>MADGGRVAQARALLQQCLHARLQVRPADGDAAAQWVEIRRGLVIYVCFFKGADTDLLPKMVNTLLNVKLSETETGKHVSILDLPGDVLIIPQATLGGRVKGRSMQYHSNSGKEEGSELYSQFVSLCEKAVANNTKSVEAGVAVAHGTYGNRQVLKLDTNGPYTHLIEF[2x]

Here, we describe the identification and characterization of a unique DTD-like factor, named Animalia-specific tRNA deacylase (ATD). Present in kingdom Animalia and more specifically all across phylum Chordata, ATD proofreads a critical tRNA selection error made by AlaRS. An unprecedented switch from the chiral-selective “Gly-cisPro” dipeptide in DTD to “Gly-transPro” in ATD is the key to ATD’s gaining of L-chiral selectivity. This “gain of function” through relaxation of substrate chiral specificity underlies ATD’s unique capability of correcting the error in tRNA selection.

To gain insights into ATD’s function, we solved the crystal structure of MmATD at 1.86 Å resolution. We were able to solve the structure by molecular replacement using PfDTD as the search model, despite the fact that the two share < 30% sequence identity. Structural superposition of MmATD on PfDTD and NTD from Pyrococcus abyssi (PabNTD) showed an r.m.s.d. of 1.68 Å over 141 Cα atoms and 3.34 Å over 77 Cα atoms, respectively. As is the case with DTD and NTD, ATD too is a homodimeric protein. The crystal structure of ATD revealed that its characteristic motifs (–PQATL– and –TNGPYTH–) are present at the dimeric interface like the corresponding active site motifs of DTD (–SQFTL– and –NXGPVT–). Surprisingly, MmATD’s Gly-Pro motif occurs in trans conformation, unlike DTD’s Gly-Pro motif which always exists in cis conformation as observed in 107 protomers of 19 crystal structures from 5 different organisms. In contrast, the interaction of MmATD’s Arg151 side chain with the main chain of Gly-transPro motif from the dimeric counterpart pulls the motif’s backbone outwards, thus holding the motif rigidly in trans conformation. Comparative analysis of active sites of DTD and ATD further revealed that the inward flip of ATD’s carbonyl oxygens due to trans conformation of its Gly-Pro motif has created “additional” space in its active site when compared to DTD. Strikingly, when tested with L-Ala-tRNAAla, 500 nM MmATD displayed noticeable activity. Strikingly, biochemical assays with MmATD showed significantly higher selectivity for the non-cognate l-Ala-tRNAThr(G4•U69) as the enzyme acts on the substrate at just 1 nM compared to its activity on the cognate l-Thr-tRNAThr(G4•U69) at 50 nM.> MATTVQLSDQSLRQLETLAIHTAHLIQPHGLVVVLQEPDLTISQISANCTGILGRSPEDLLGRTLGEVFDSFQIDPIQSRLTAGQISSLNPSKLWARVMGDDFVIFDGVFHRNSDGLLVCELEPAYTSDNLPFLGFYHMANAALNRLRQQANLRDFYDVIVEEVRRMTGFDRVMLYRFDENNHGDVIAEDKRDDMEPYLGLHYPESDIPQPARRLFIHNPIRVIPDVYGVAVPLTPAVNPSTNRAVDLTESILRSAYHCHLTYLKNMGVGASLTISLIKDGHLWGLIACHHQTPKVIPFELRKACEFFGRVVFSNISAQEDTETFDYRVQLAEHEAVLLDKMTTAADFVEGLTNHPDRLLGLTGSQGAAICFGEKLILVGETPDEKAVQYLLQWLENREVQDVFFTSSLSQIYPDAVNFKSVASGLLAIPIARHNFLLWFRPEVLQTVNWGGDPNHAYEATQEDGKIELHPRQSFDLWKEIVRLQSLPWQSVEIQS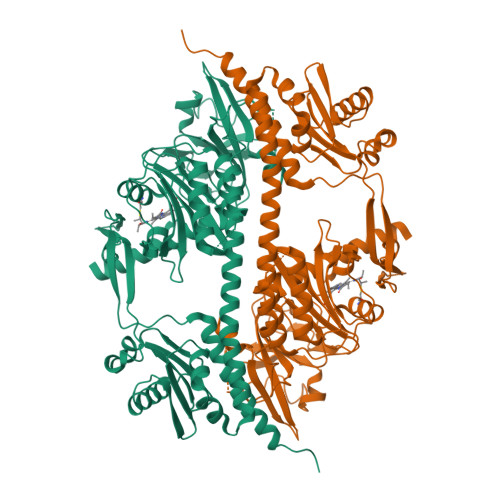ALALKKAIVNLILRQAEEHHHHHH> SNAMIYPYKEKKPKIASSAFIADYVTITG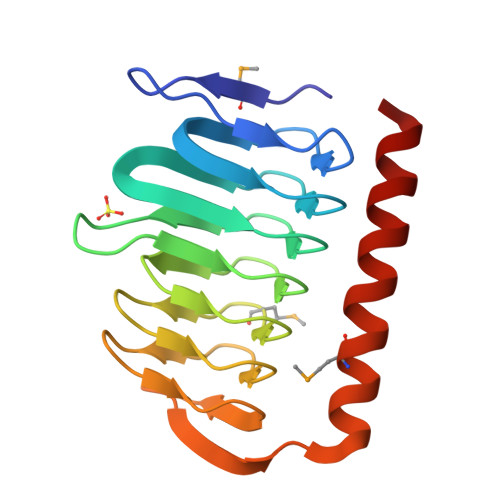DVYVGEESSIWFNTVIRGDVSPTIIGDRVNVQDQCTLHQSPQYPLILEDDVTVGHQVILHSCHIKKDALIGMGSIILDGAEIGEGAFIGAGSLVSQGKKIPPNTLAFGRPAKVIRELTAEDRKDMERIRTQYVEKGQYYKSLQK>[2x]ATELDVDGVKVRFTNPDKVYFPKLGKNGTKGKLVEYYLSVASGPMLALLRDRPVHLQRFPDGIEGEEIYQKRVPQKHPDYLETCVVTFPSGRTADALKITHPSSIIWAAQMGTVTLHPWQVRCPDTEHPDELRVDLDPQPGTGFKEARTVACDVLKPLLDELGLVGYPKTSGGRGVHVFLRIKPQWDFIEVRRAGIALAREVERRAPDAVTTSWWKEERGERLFIDYNQNARDRTFASAYSVRKTPIATVSMPLSWDELRNADPDDYTMNTVPDLLAGRDDPWADIDSVQQSLGPLLDLVAADEERGLGDLPYPPNYPKMPGEPPRVQPSK

One orthologue, MSMEG_6301 (Prim-PolC/LigC Pol/PolD) is encoded in the genomic proximity of two DNA ligase genes (LigC1: msmeg_6302 and LigC2: msmeg_6304). We show that components of the LigC complex act together to preferentially fill in short DNA gaps with ribonucleotides (rNTPs), followed by sealing of the resulting nicks. LigD-deficient cells are also sensitive to oxidative damaging agents, uncovering an unexpected duel role in both excision and DSB repair. Together, these findings establish that the LigC complex operates in excision repair pathways that specifically mends lesions and single-strand breaks in stationary phase. Prim-PolC preferentially binds to and fills-in short DNA gaps.

To define molecular differences between these distinct Prim-Pols, we elucidated the crystal structure of Ms Prim-PolC and compared it to a NHEJ-specific Prim-Pol. Prim-PolC retains the same overall fold of the mycobacterial Prim-PolD (PolDom) structure, which can be superposed with an RMSD of 1.712 Å (over 270 aligned positions, Fig. 5a). Shared structural features include the phosphate recognition pocket containing the conserved basic residues (K23, K35 and N20) that facilitate this key DNA interaction. Despite these similarities, Prim-PolC orthologues possess a strictly conserved C-terminal extension whose function has not been ascribed. In the Prim-PolC structure, we observe that this additional C-terminal region (aa 294–336) consists of a conserved alpha helix (residues G299−R311), which lies across alpha helix 4 after which the peptide chain becomes an unstructured loop. Notably, this structural element, termed Loop 3 (residues G313−P333), is positioned between the two prominent surface loops (1 and 2) that together form a continuous surface on one side of the active site pocket. Apical Loop 1 residues, normally involved in template strand orientation, are not conserved and are instead repurposed for locking Loop 3 into position. Residue P94 packs against a pocket formed of residues Y321, P322, K323 and M324 from Loop 3. Loop 2 residue W219 interacts with Loop 3 residues P316, Y317, P333 and K335 via a mixture of hydrophobic and polar interactions. Again, this has the effect of locking Loop 3 into its current orientation, and also reorients Loop 2 into a more distal position to the active centre, compared to the existing Prim-PolD MMEJ structure.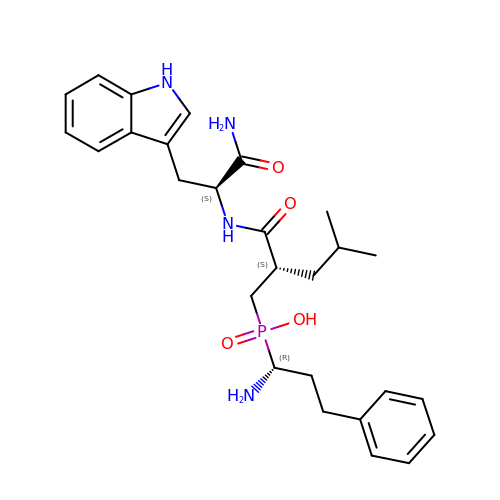Nalpha-[(2S)-2-{[[(1R)-1-amino-3-phenylpropyl](hydroxy)phosphoryl]methyl}-4-methylpentanoyl]-L-tryptophanamide | C27 H37 N4 O4 P | QKFOTLXPIIESQI-IEZKXTBUSA-N> MARDPLPFFPPLYL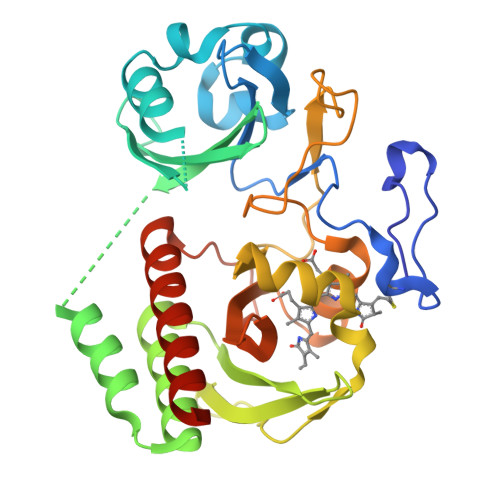GGPEITTENCEREPIHIPGSIQPHGALLTADGHSGEVLQVSLNAATFLGQEPTVLRGQTLAALLPEQWPALQAALPPGCPDALQYRATLDWPAAGHLSLTVHRVAELLILEFEPTEAWDSIGPHALRNAMFALESAPNLRALAEVATQTVRELTGFDRVMLYKFAPDATGEMIAEARREGMQAFLGHRFPASHTPAQARALYTRHLLRLTADTRAAAVPLDPVLNPQTNAPTPLGGAVLRATSPMHMQYLRNMGVGSSLSVSVVVGGQLWGLIVCHHQTPYVLPPDLRTTLEYLGRKLSGQVQRKEAEFHHHHHH>[2x]GSPASGTSLSAAIHRTQLWFHGRISREESQRLIGQQGLVDGLFLVRESQRNPQGFVLSLCHLQKVKHYLILPSEEEGRLYFSMDDGQTRFTDLLQLVEFHQLNRGILPCLLRHCCTRVAL;>[2x]SFEGYDNXFPX

Growth factor receptor-bound protein 7 (Grb7) is an adaptor protein involved in cell signaling where it interacts with a number of tyrosine kinases via its src-homology2 (SH2) domain78. In this way it plays a role in integrin dependant cell migration via its interaction with focal adhesion kinase and subsequent phosphorylation in focal contacts, consistent with its homology to the C. Elegans protein Mig-10 that is involved in cellular migration. It has been shown that overexpression of Grb7 enhances cell migration, while inhibition of Grb7 lowers the migratory potential of cells and is therefore linked with metastatic spread of cancer cells. While co-overexpression of Grb7 and ErbB2 occurs due to the proximity of their two genes on the 17q12-21 amplicon, Grb7 plays a role independent of ErbB2 in cancer progression. These important roles of Grb7 in numerous cancers have established Grb7 as a therapeutic target. Following the conventional nomenclature for SH2 domains, the Grb7-SH2 domain possesses a 3 stranded anti-parallel β-sheet consisting of the βB, βC and βD strands, flanked by 2 α-helices, αA and αB.

Here we report the crystal structure of G7-B1 in complex with Grb7-SH2 domain, revealing an unanticipated mode of binding involving interactions between the staple and Grb7-SH2 domain. The asymmetric unit consists of two Grb7-SH2 domains (with residues 426–528 in chain A and 424–527 in chain B visible in the electron density), two G7-B1 peptides, 171 water molecules, and two phosphate anions that are positioned in the phosphotyrosine binding site of each Grb7-SH2 monomer. The immediate striking feature of the G7-B1 interaction with the Grb7-SH2 domain is that, instead of the staple acting as a stabilising tether, it acts to form a new Grb7-SH2 domain interaction surface. While the amino acid residues 2–7 are positioned as expected from our knowledge of the G7-18NATE interaction, residues 9, 10 and 11 no longer interact at the surface of the protein but form a loop that sits above the staple away from the protein surface. Y5 is positioned in the pY binding site precisely as seen in the G7-18NATE structure forming hydrogen bonds with Asn463(ND2) and Ser460(OG) in the BC loop of Grb7-SH2. Additionally the Y5 of G7-B1 forms a hydrogen bond with the phosphate anion bound to the Grb7-SH2 domain, together effectively mimicking the presence of a pY. G7-B1 is further stabilised by hydrogen bonds and a salt bridge between E3(OE1 and OE2) and Arg 462(NH1 and NH2) with these interactions not previously seen in Grb7-SH2/peptide structures. Instead the staple forms close contacts with Met 495, Asp 496, Asp 497 mainchain and sidechain atoms in the EF loop of Grb7-SH2 and Ile 518 sidechain in the BG loop. The staple contributes 83 Å2 of the total interaction surface area of 548 Å2.>IVGGKDAPVGKYPYQVSLRLSGSHRCGASILDNNNVLTAAHCVDGLSNLNRLKVHVGTNYLSESGDVYDVEDAVVNKNYDDFLLRNDVALVHLTNPIKFNDLVQPIKLS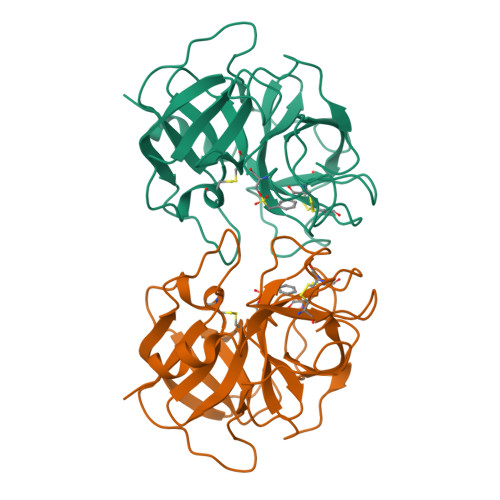TNDEDLESNPCTLTGWGSTRLGGNTPNALQEIELIVHPQKQCERDQWRVIDSHICTLTKRGEGACHGDSGGPLVANGAQIGIVSFGSPCALGEPDVYTRVSSFVSWINANLKK[2x]>MSNISLIVGLGNPGSEYAQTRHNAGFWFVEQLADKYGITLKNDPKFHGISGRGNIEGHDVRLLLPMTYMNRSGQSVVPFSKFYQIAPEAILIAHDELDMNPGVIRLKTGGGHGGHNGLRDIVPHIGPNFHRLRIGIGHPG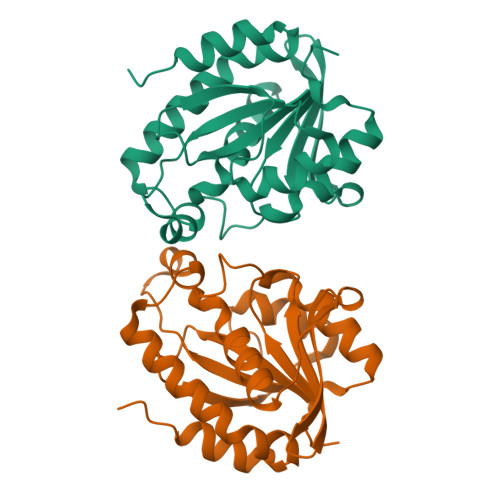SKERVSGHVLGKAPSNEQSLMDGAIDHALSKVKLLVQGQVPQAMNQINAYKPA[2x]> GSMPLLLDDGDPKAQTGFDLSTATTLFWRPVPVHVKQQDREDVLEELTFRILTGVAKQNHNLRILRIHISSDS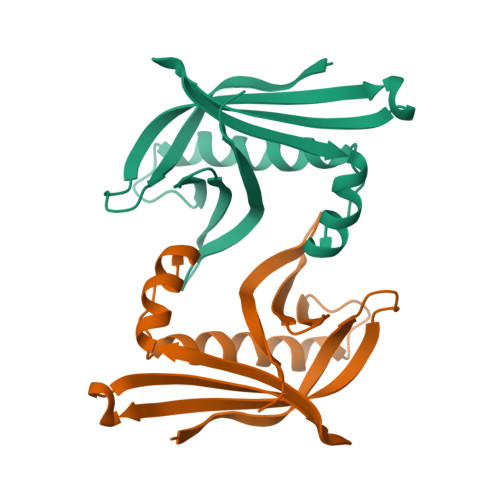DLFFLHTLEVSEEDFQSLKNDEGILVDFASFPGKIISLLEKCILAQPGDSPRFQAVLTIRGGESVFKIVEINDWRQLPHITLAFRPGN> MAATTVNGGTVHFKGEVVNAACAVDAGSVDQTVQLGQVRTASLAQEGATSSAVGFNIQLNDCDTNVASKAAVAFLGTAIDA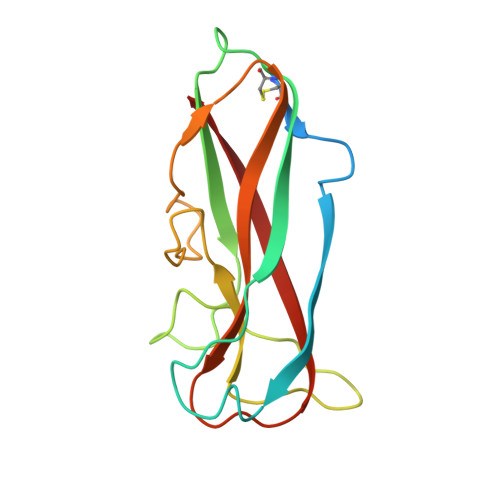GHTNVLALQSSAAGSATNVGVQILDRTGAALTLDGATFSSETTLNNGTNTIPFQARYFATGAATPGAANADATFKVQYQ>[4x]MRGSHHHHHHGSLVPRGS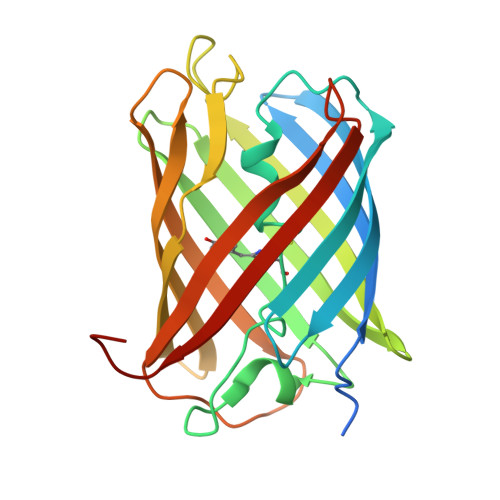MVSVIKPDMKIKLRMEGAVNGHPFAIEGVGLGKPFEGKQSMDLKVKEGGPLPFAYDILTTVFCYGNRVFAKYPENIVDYFKQSFPEGYSWERSMNYEDGGICNATNDITLDGDCYIYEIRFDGVNFPANGPVMQKRTVKWEPSTEKLYVRDGVLKGDVNMALSLEGGGHYRCDFKTTYKAKKVVQLPDYHFVDHHIEIKSHDKDYSNVNLHEHAEAHSELPRQAK> NALRRDPNLPVHIRGWLHKQDSSGLRLWKRRWFVLSGHCLFYYKDSREESVLGSVLLPSYNIRPDGPGAPRGRRFTFTAEHPGMRT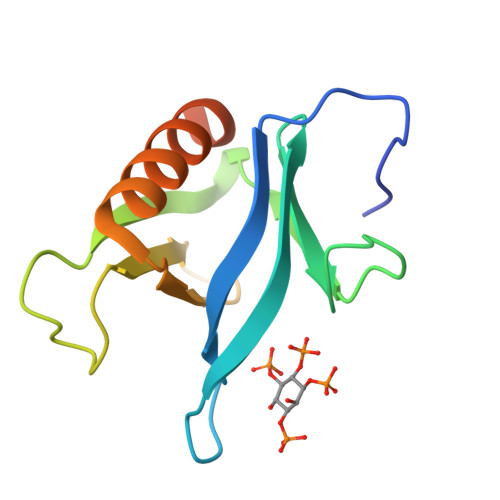YVLAADTLEDLRGWLRALGRASRAEGDDYGQPRSPAR3-NITROTOLUENE 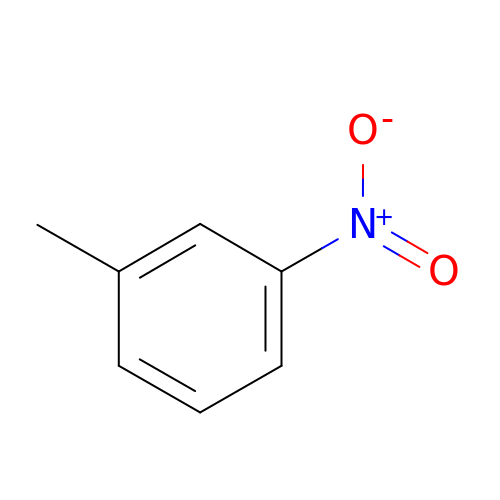| C7 H7 N O2 | QZYHIOPPLUPUJF-UHFFFAOYSA-N>NLNKRMGDLRDINGEAGAWARIMSGTGSASGGFSDNYTHVQVGVDKKHELDGLDLFTGFTVTHTDSSASADVFSGKTKSVGAGLYASAMFDSGAYIDLIGKYVHHDNEYTATFAGLGTRDYSTHSWYAGAEAGYRYHVTEDAWIEPQAELVYGSVSGKQFAWKDQGMHLSMKDKDYNPLIGRTGVDVGKSFSGKDWKVTARAGLGYQFDLLANGETVLRDASGE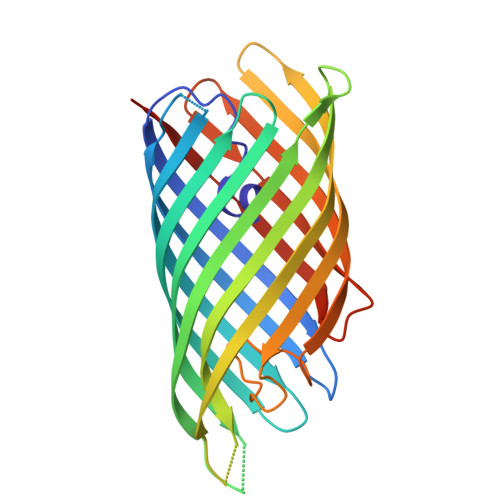KRIKGEKDSRMLMSVGLNAEIRDNVRFGLEFEKSAFGKYNVDNAVNANFRYSFGSHHHHHH[2x]>[2x]MGSSHHHHHHSQDPGDENLYFQSMSDADRIAALLKDRAADPVTKFSPSPYETGQFLRISERADVGTPQIDYLLATQRPDGLWGSVGFELVPTLGAVAGLSSRPEYADRAGVTDAVARACEKLWELALGEGGLPRLPDTVASEIIVPSLIDLLGEVLQRHRPAAGGKAGHEQEFPSPPGAKPELWRRLSDRIARGQAIPETAWHTLEAFHPLPEQFAATVTPAADGAVTCSPSSTAAWVSAVGTDAGASTRAYLDEAQSRYGGAIPMGSSMPYFEVLWVLNLVLKYFPDVPIPREIIEEIAAGFSESGIGGGPGLPPDGDDTAYANLAGDKLGAPTHPEILMKFWAEDHFVSYPGEQTPSETVNAHALEYLNHLRLRRGIAEYGAVEDACAEWVISQQTEDGCWYDKWNVSPYYSTAACVEALLDARKQDEPQLDSLRRAREWLLRHQTDSGGWGMAEPSPEETAYAVMALDLFASRGGKGAEECAAAISRAKEFFKDESRENPPLWMGKDLYTPFRIVEVTVMCGRAVVSRY

To contribute towards understanding the sequence-structure-function relationships of type II bacterial TSs, we determined the structure of the terpentedienyl diphosphate synthase Tpn2 from Kitasatospora sp. CB02891 by X-ray crystallography and made structure-guided mutants to probe its mechanism. TSs employ carbocation chemistry to convert acyclic prenyl diphosphates into diverse terpene skeletons. Canonical bacterial TSs are categorized into type I or type II depending on how they initiate catalysis.

We experimentally verified Tpn2 as a TPP synthase and determined its structure by X-ray crystallography at a resolution of 2.57 Å. This is only the third structurally determined bacterial type II TS and the first from any organism that produces a clerodane skeleton. As seen in PtmT2 and Rv3377c16,26, Tpn2 adopts the characteristic double α-barrel βγ fold with the active site residing in the interfacial cavity. As is typical for TSs from both eukaryotes and prokaryotes, the active site cavity of Tpn2 is lined with both aromatic (H180, F250, W254, Y329, W384, W483, and Y489) and aliphatic (V116, A117, T177, T181, G244, G287, L291, and G485) residues to form a hydrophobic pocket suitable for binding the long nonpolar tail of the substrate and preventing water or other nucleophiles from prematurely quenching the reaction. At the bottom of the active site pocket lies the catalytically essential Asp-rich motif D294xDD. Docking experiments support that the central Asp, D296, is properly positioned (3.2 Å from C14) for both the protonation of GGPP and the deprotonation of the syn-cleroda-13E-en-4-yl+ intermediate (TPP+). D296 is also suitably positioned (2.8 Å) near H342 for activation. As with PtmT2 and Rv3377c, no bound divalent metal ions can be inferred in the electron density of the crystal structure of Tpn2, leaving the exact binding mechanism of divalent ions in bacterial type II TSs undetermined. Lacking an analogous Asp on the side opposing the DxDD motif, Tpn2 instead has a G485 situated 3.6 Å from C19 of the substrate. Thus, G485D acts as a single-residue switch, exhibiting sole control over the formation of the clerodane TPP or labdane syn-CPP.> AGAGGAGAUCUCCUCU

To further understand the structure and properties of the D:U base pair and the D:C mismatch, we designed and synthesized self-complementary RNA sequences that form duplexes with two separated or adjacent D:U or D:C pairs. All four oligonucleotides crystallized within 2–3 days at 20 °C under their optimal crystallization conditions, and we solved their structures by X-ray diffraction at a resolution higher than 1.65 Å. We found that all four structures adopt the same space group (R32). Each unit cell contains only a single RNA strand so that each duplex features two identical D-containing base pairs.

The sequence UD-1, 5′-AGA GDA GAU CUU CUC U-3′, can form two separated D:U pairs with the underlined nucleobases, while the sequence CD-1, 5′-AGA GDA GAU CUC CUC U-3′, can form two separated D:C pairs. Examination of the crystal structures of the CD-1 and CD-2 duplexes shows that the D:C mismatches all adopt the classical wobble base pair geometry that is isomorphic with a G:U wobble pair. The N6–N3 and N1–O2 distances are similar for CD-1 and CD-2 duplexes: 2.9 Å vs 2.8 and 2.8 Å vs 2.7 Å. Based on the observed interatomic distances, the D:C pairs in the CD-1 and CD-2 duplexes appear to have two hydrogen bonds: N6–N3 and N1–O2. However, an N1–O2 hydrogen bond requires N1-protonation of D in D:C pairs. Solution-phase NMR studies revealed that the 2-aminopurine (2AP)-cytosine (C) pair exists predominantly as a protonated pair as opposed to an imino tautomer at physiological pH. Since D has an additional electron-donating amino group, N1 in D has a higher pKa value and is more likely to be protonated than N1 in 2AP. Therefore, D in the D:C pairs likely exists as a protonated D in the canonical amino tautomeric form. Crystallographic studies reveal that the protonated amino form of D can form a base pair with C that is isostructural to a G:U wobble pair, which may account for the increased rate of D:C mismatches in the defined construct. Therefore, D:C mismatches have a strong stalling effect on downstream primer extension.N-(4-(dibenzylamino)-4-oxobutyl)-2-(5-(dimethylamino)pentanamido)-4-methylpentanamide 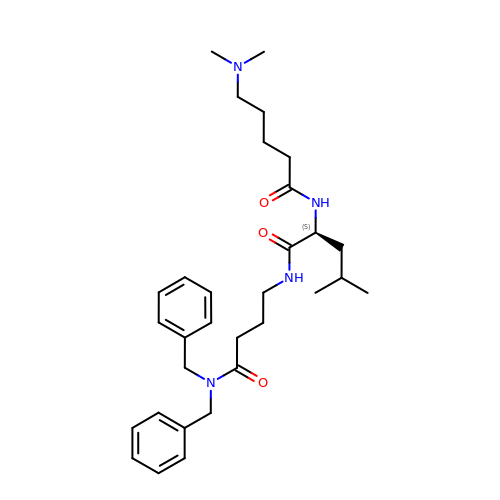| C31 H46 N4 O3 | MYOVPOSHNFZORZ-NDEPHWFRSA-N>MDTPNKDDSIIRFSVSLQQNLLDELDNRIIKNGYSSRSELVRDMIREKLVEDNWAEDNPNDESKIAVLVVIYDHHQRELNQRMIDIQHASGTHVLCTTHIHMDEHNCLE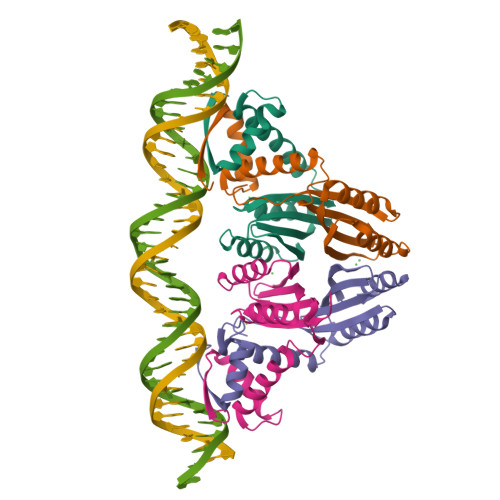TIILQGNSFEIQRLQLEIGGLRGVKFAKLTKASSFEYNE[4x]> QPVVKSLLNSKGIHYNQGNPYNLLTPVIEKVKPGEQSFVGQHAATGCVATATAQIMKYHNYPNKGLKDYTYTLSSNNPYFNHPKNLFAAIS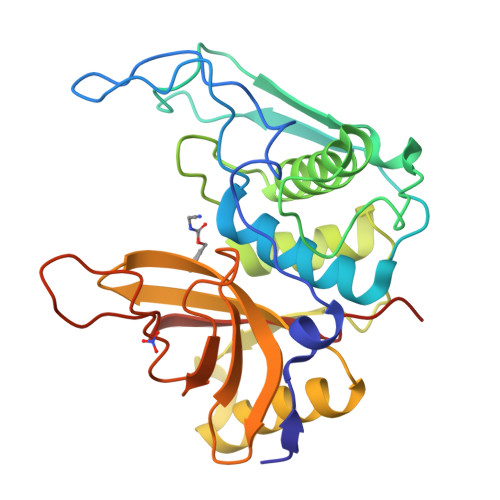TRQYNWNNILPTYSGRESNVQKMAISELMADVGISVDMDYGPSSGSAGSSRVQRALKENFGYNQSVHQINRSDFSKQDWEAQIDKELSQNQPVYYQGVGKVGGHAFVIDGADGRNFYHVNWGWGGVSDGFFRLDALNPSALGTGGGAGGFNGYQSAVVGIKPLEHHHHHH>[2x]MGSDKIHHHHHHENLYFQGMRISANFDGGNIETISLANPDDIQLAIRPDAGGEFYQWFNFRFEATIGKTYTLNILNAGGASYLKGWEDYQAVASYDRQTWFRLPTEYKDGKLSISVELDCEAIQIAYFTPYSYERHLDLISAVQLHPLVST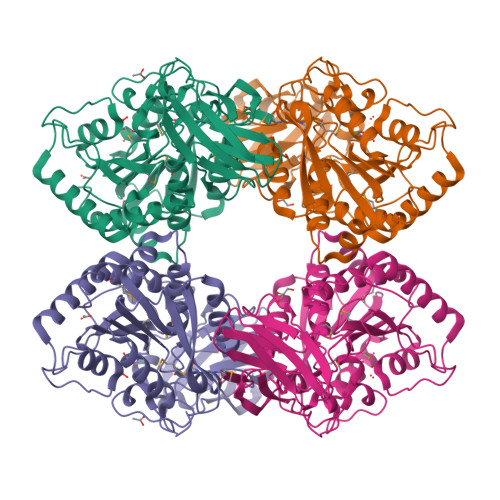EHLGLTLDGRDMTLVKVGDDDPSKKSIWITARQHPGETMAEWLVEGLLNQLLDNDCPTSKALLDKANFYIVPNMNPDGSVRGHLRTNAVGANLNREWQTPSLERSPEVYYVVNKMHETGVDLFYDVHGDEGLPYVFLAGCEGIPNYSDKLASLQQDFVAALSLASADFQTEFGYDKDEPGKANLTVACNWVANTFKCLSNTLEMPFKDNANLADPFQGWSPERSVYFGEASLIAMRAVIDKIGQ> MRLYCLSGDLAKPCYIITFKGLRIMLDCGLTEQTVLNFLPLPFVQ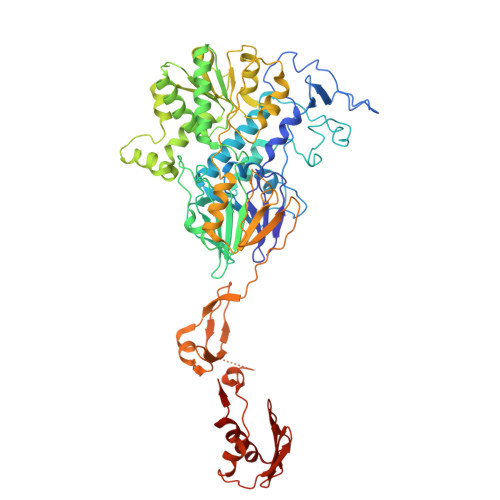SLKWSNLPNFVPSRDHDPQMDGELKDCCGRVFVDSTPEFNLPMDKMLDFSEVDVILISNYLNMLALPYITENTGFKGKVYATEPTLQIGRFFLEELVDYIEVSPKACTARLWKEKLHLLPSPLSEAFRAKKWRTIFSLKDVQGSLSKVTIMGYDEKLDILGAFIATPVSSGYCLGSSNWVLSTAHEKICYVSGSSTLTTHPRPINQSALKHADVLIMTGLTQAPTVNPDTKLGELCMNVALTIRNNGSALIPCYPSGVVYDLFECLTQNLENAGLNNVPMFFISPVADSSLAYSNILAEWLSSAKQNKVYLPDDPFPHAFYLRNNKLKHYNHVFSEGFSKDFRQPCVVFCGHPSLRFGDAVHFIEMWGNNPNNSIIFTEPDFPYLQVLAPFQPLAMKAFYCPIDTSLNYQQANKLIKELKPNVLVIPEAYTKPHPSAPNLFIEQPDKKIITFKCGEIIRLPLKRKLDRIYITSELAQKISPKEVAAGVTFSTLTGVLQVKDKVHCIQPCADSVKDETISSNSAPTKEDVLKNVKYEYGSIDVDAVMKKLAQDGFSNIKLDRTGGALTLNLVNEDTVIKFEDNETHIICGGKPTTRLKLRDTIMKCLQSF In siphophage T5, the unique RBP is located at the extremity of a central fiber. FhuA, an outer membrane E. coli iron-ferrichrome transporter, is the bacterial receptor recognized by T5 (25). We present the structures of T5 tail tip, determined by cryo–electron microscopy before and after interaction with its E. coli receptor, FhuA, reconstituted into nanodisc. These structures bring out the important conformational changes undergone by T5 tail tip upon infection, which include bending of T5 central fiber on the side of the tail tip, tail anchoring to the membrane, tail tube opening, and formation of a transmembrane channel.

When comparing the structures of the tip before and after interaction with FhuA, we could observe that they share a common core from the tail tube down to BHPpb3 and only start to diverge from BHPpb3 distal part. Our tail tip structure includes two TTPpb6 rings that could be modeled. The tube extends through the tip: After the last TTPpb6 ring, it continues with a pseudo-hexameric p140 ring, a hexameric DTPpb9 ring, the proximal domains of the BHPpb3 trimer forming the last pseudo-hexameric ring of the tube. Thus, the tube diameter is conserved, although the pitch and the twist between the different rings are different. The p140 ring is surrounded by a larger p132 dodecameric ring, p140 C terminus making direct contacts with a p132 monomer, explaining the need for a decoration-less ring at this position. The collar is made of a dodecamer of p132, whose position and structure were previously unknown. The dodecameric p132 ring completely surrounds the trimeric p140 ring, with p132-p132 and p132-p140 contacts in both p132 and p140 proximal regions and, to a much lesser extent, p132-TTPpb6 contacts, mainly mediated through the loops and termini of the three proteins. Here, however, the DTPpb9 ring is sandwiched between two threefold symmetric rings (TTPpb6 and BHPpb3), which both have a pseudo-sixfold symmetry. There is a symmetry mismatch between LTFpb1 3-fold, p140/TTPpb6 pseudo–6-fold, and p132 pseudo–12-fold symmetries. This symmetry mismatch is absorbed by the loops and N termini of p132 monomers.

>[6x]MSLQLLRNTRIFVSTVKTGHNKTNTQEILVQDDISWGQDSNSTDITVNEAGPRPTRGSKRFNDSLNAAEWSFSTYILPYKDKNTSKQIVPDYMLWHALSSGRAINLEGTTGAHNNATNFMVNFKDNSYHELAMLHIYILTDKTWSYIDSCQINQAEVNVDIEDIGRVTWSGNGNQLIPLDEQPFDPDQIGIDDETYMTIQGSYIKNKLTILKIKDMDTNKSYDIPITGGTFTINNNITYLTPNVMSRVTIPIGSFTGAFELTGSLTAYLNDKSLGSMELYKDLIKTLKVVNRFEIALVLGGEYDDERPAAILVAKQAHVNIPTIETDDVLGTSVEFKAIPSDLDAGDEGYLGFSSKYTRTTINNLIVNGDGATDAVTAITVKSAGNVTTLNRSATLQMSVEVTPSSARNKEVTWAITAGDAATINATGLLRADASKTGAVTVEATAKDGSGVKGTKVITVTAGG;>MFYSLMRESKIVIEYDGRGYHFDALSNYDASTSFQEFKTLRRTIHNRTNYADSIINAQDPSSISLAINFSTTLIESNFFDWMGFTREGNSLFLPRNTPNIEPIMFNMYIINHNNSCIYFENCYVSTVDFSLDKSIPILNVGIESGKFSEVSTFRDGYTITQGEVLPYSAPAVYTNSSPLPALISASMSFQQQCSWREDRNIFDINKIYTNKRAYVNEMNASATLAFYYVKRLVGDKFLNLDPETRTPLIIKNKYVSITFPLARISKRLNFSDLYQVEYDVIPTADSDPVEINFFGERK[3x];>MSTENRVIDLVVDENVPYGLLMQFMDVDDSVYPSTSKPVDLTDFSLRGSIKSSLEDGAETVASFTTAIVDAAQGVASISLPVSAVTTIASKASKERDRYNPRQRLAGYYDVIITRTAVGSAASSFRIMEGKVYISDGVTQ[12x];>[6x]MRLPDPYTNPEYPGLGFESVNLVDNDPMIRDELPNGKVKEVKISAQYWGINISYPELFPDEYAFLDSRLLEYKRTGDYLDVLLPQYEAFRVRGDTKSVTIPAGQKGSQIILNTNGTLTGQPKAGDLFKLSTHPKVYKITNFSSSGNVWNISLYPDLFITTTGSEKPVFNGILFRTKLMNGDSFGSTLNNNGTYSGISLSLRESL COUMARIN | C9 H6 O2 | 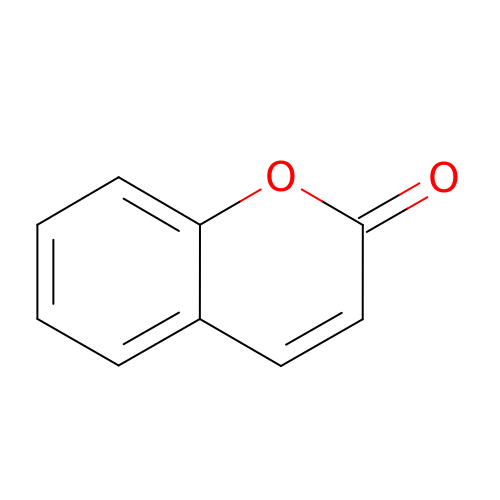ZYGHJZDHTFUPRJ-UHFFFAOYSA-N In most bacteria and eukaryotes, queuosine (Q) is universally found at the wobble position (position 34) of four specific tRNAs featuring “GUN” anticodon sequences, namely tRNATyrGUA, tRNAAspGUC, tRNAAsnGUU, and tRNAHisGUG7,8. Prokaryotes can synthesize Q from GTP de novo, whereas eukaryotes need to salvage the modified nucleoside or the base queuine (q) from their diet and microbiota. In eukaryotes, the incorporation of q into tRNAs is carried out by the tRNA guanine transglycosylase complex (TGT), comprising the catalytic queuine tRNA-ribosyltransferase subunit 1 (QTRT1), and the accessory subunit QTRT2. The Q modification at the wobble position increases the efficiency of decoding during translation.

Structures of mouse QTRT1/2 in complex with mature tRNATyr and pre-tRNATyr by single particle cryo-Electron Microscopy (cryo-EM) confirm that the complex is able to bind both forms in an almost identical fashion. Next, we prepared cryo-EM grids with the purified mQTRT1/2 in the presence of 9dG and either mature tRNATyr or the pre-tRNATyr 1-4. After additional 3D classification and refinement routines, final maps at an overall resolution of 2.9 Å (mQTRT1/2-tRNATyr) and 3.1 Å (mQTRT1/2-pre-tRNATyr 1-4), respectively, were obtained. The cryo-EM structure of mouse QTRT1/2 reveals the heterodimeric organization of the complex accommodating tRNA that resembles the previously described apo crystal structures of mouse and human QTRT1/2 in complex with tRNAAsp12. Foremost, the structures show that mouse QTRT1/2 binds tRNATyr and the intron-containing pre-tRNATyr 1-4 in an almost identical fashion as human QTRT1/2 binds tRNAAsp12. QTRT1 binds and rearranges the anticodon stem loop (ASL) of the mature as well as the pre-tRNA to accommodate the modified position 34 in the active site. QTRT2 contributes to tRNA binding by contacting the D-loop and the acceptor stem. The 9dG molecule is visible in the active sites of both structures, which show an overall r.m.s.d.698 residues of 1.13 Å. In summary, our cryo-EM structures confirm that mouse QTRT1/2 is able to accommodate both mature as well as precursor tRNATyr and that G34 is positioned correctly in the active site to accomplish the G-to-Q exchange reaction, regardless of the presence of the intronic sequence.

> GPESAPRIMRLVAECSRSGARAGELRLPHGTVATPVFMPVGTQATMKGITTEQLDSLGCRICLGNTYHLGLRPGPELIRKAQGLHGFMNWPHNLLTDSGGFQMVSLFSLSEVTEEGVHFRSPYDGEETLLSPERSVEIQNALGSDIIMQLDHVVSSTVTGPLVEEAMHRSVRWLDRCIAAHKHPDKQNLFAIIQGGLNADLRTTCLKEMTKRDVPGFAIGGLSGGESKAQFWKMVALSTSMLPKDKPRYLMGVGYATDLVVCVALGCDMFDCVYPTRTARFGSALVPTGNLQLKKKQYAKDFSPINPECPCPTCQTHSRAFLHALLHSDNTTALHHLTVHNIAYQLQLLSAVRSSILEQRFPDFVRNFMRTMYGDHSLCPAWAVEALASVGIMLT;> GPKLSLIKVVNGCRLGKIQNLGKAGDCTVDIPGCLLYTRTGSAPHLTHQTLRNIHGVPGIAQLTLSSLAEHHEVLAEYKKGVGSFIGMPESLFYCSLHDPVTPGPAGYVTSKSVSVWGFGGRVEMTVSKFMAIQEALQPDWFQCLSDGEASCAETTSIKRARKSVDRSLLFLDSCLRLQEESEVLQKSVIIGVIEGGDVMEERLRSARETAKRPVGGFLLDGFQGDPAVTETRLHLLSSVTAELPEDKPRLICGVSRPDEVLECIERGVDLFESFFPYQVTERGCALTFTFDCQLNPEETLLQQNGIQEKIKGLDQAKKIEATGCNQEMTSFEINLKEKKYQEDFDPLVRGCSCYCCKNHTRAYIHHLLMTNELLAGVLLMMHNFEHYFGFFCSIREALKNDTLAQLKELICRQMF>GSKGRLVIYCSATNVMCENAAKTFEQKYDVKTSFIRNGSGSTFAKIEAEKNNPQADVWYGGTLDPQSQAGELGLL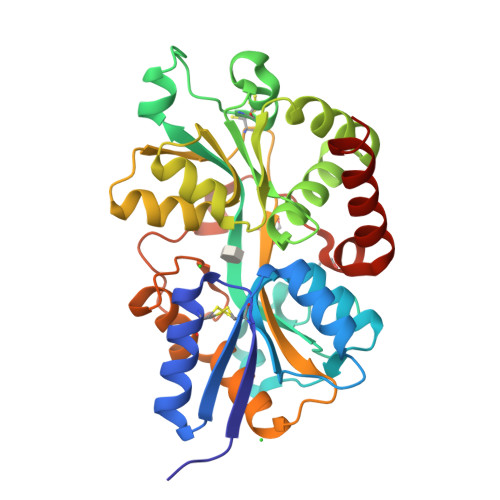EAYRSPNIDQIMPKFQDPAKVKGNLSSAVYIGILGFAVNTERLKKLGIEKIPQCWNDLTDPKLKGEIQIADPQSSGTAYTAIATFAQLWGEDKAFDYFKHLHPNISQYTKSGITPARNAARGETTVGIGFLHDYALEKEQGAPLEMVVPCEGTGYELGGVSILKGARNLDNAKLFVDFALSKEGQETAWKKGQALQTLTNTTAEQSPLAFDLTKLKLIDYDFEKYGASDERKRLINKWVDEIKLAK[2x]>SNAQEQRMSHHYATIEVSQQLRQLLGDQLVILLRETPDGQALERSQNDFRRVLEQGRANTVDSAEQAALDGVRDAYLQLQAHTPALLEAPMADNDGFSEAFNGLRLRL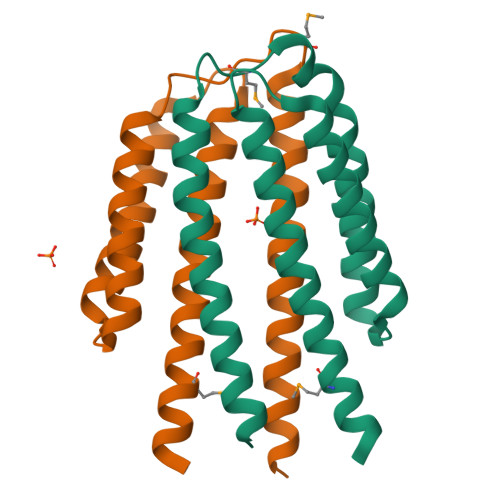QDLQQLALAGISEAETSARHRA[2x]>[2x]MSWENPGPPKRADARRNYDRIIEAAAAEVARHGADASLEEIARRAG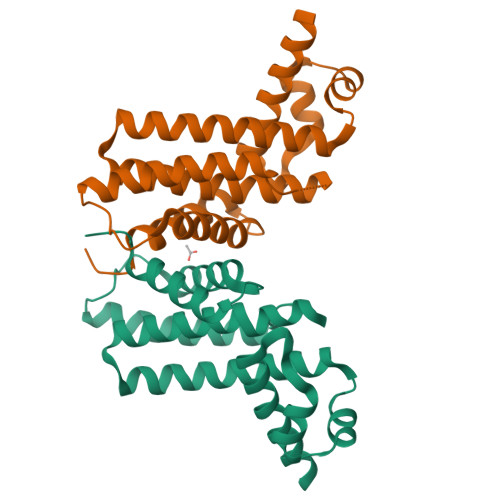VGSATLHRHFPSRWGLLQAVFQERVAQLCDEARSLAAEHPPATALTRWLTSLAVFGAVTRGAARSLLPATGTNTGAALDSRCEQLLTEAGADLLARAQEDGTVRDDVTALELLSLANAVSLAAEHTPDAAHHATRLMGIALGGLGAPGPRPQG>MAQVINTNSLSLLTQNNLNKSQSALGTAIERLSSGLRINSAKDDAAGQAIANRFTANIKGLTQASRNANDGISIAQTTEGALNEINNNLQRVRELAVQSANSTNSQSDLDSIQAEITQRLNEIDRVSGQTQFNGVKVLAQDNTLTIQVGANDGETIDIDLKQINSQTLGLDTLNVQQKYKVSDTAATVTGYADTTIALDNSTFKASATGLGGTDQKIDGDLKFDDTTGKYYAKVTVTGGTGKDGYYEVSVDKTNGEVTLAGGATSPLTGGLPATATEDVKNVQVANADLTEAKAALTAAGVTGTASVVKMSYTDNNGKTIDGGLAVKVGDDYYSATQNKDGSISINTTKYTADDGTSKTALNKLGGADGKTEVVSIGGKTYAASKAEGHNFKAQPDLAEAAATTTENPLQKIDAALAQVDTLRSDLGAVQNRFNSAITNLGNTVNNLTSARSRIEDSDYATEVSNMSRAQILQQAGTSVLAQANQVPQNVLSLLR[17x];>MASISSLGVGSNLPLDQLLTDLTKNEKGRLTPITKQQSANSAKLTAYGTLKSALEKFQTANTALNKADLFKSTVASSTTEDLKVSTTAGAAAGTYKINVTQLAAAQSLATKTTFATTKEQLGDTSVTSRTIKIEQPGRKEPLEIKLDKGDTSMEAIRDAINDADSGIAASIVKVKENEFQLVLTANSGTDNTMKITVEGDTKLNDLLAYDSTTNTGNMQELVKAENAKLNVNGIDIERQSNTVTDAPQGITLTLTKKVTDATVTVTKDDTKAKEAIKSWVDAYNSLVDTFSSLTKYTAVEPGEEASDKNGALLGDSVVRTIQTGIRAQFANSGSNSAFKTMAEIGITQDGTSGKLKIDDDKLTKVLKDNTAAARELLVGDGKETGITTKIATEVKSYLADDGIIDNAQDNVNATLKSLTKQYLSVSNSIDETVARYKAQFTQLDTMMSKLNNTSSYLTQQFTAMNKS[5x]

The flagellum is the most prominent extracellular structure in bacteria, with a molecular weight in the hundreds of megadaltons. Structurally, the flagellum can be divided into three major components: basal body, hook and filament. A ring-like structure formed by the proteins FlgK and FlgL, termed the hook–filament junction (HFJ), forms the connection between the flexible hook and the rigid filament. To assemble a filament, flagellin monomers are secreted through the flagellar basal body and hook, and polymerize at the distal end.

Here we report the structure of the filament cap complex in its native environment, assembled at the distal end of the flagellar filament. Three-dimensional (3D) classification identified the different states of the cap, resulting in a final 3.7-Å map resolving all five FliD subunits. The final cap model contains 5 FliD subunits and 17 copies of FliC in the filament; the HFJ model contains 13 copies of FlgE, 11 copies of FlgK and FlgL, and 14 copies of FliC. The flagellar cap complex is composed of five FliD subunits assembled into a pentamer with an overall shape resembling an acorn. The D2–D3 domains assemble into a star-shaped plane and the D0–D1 helices form a plug-like structure beneath. The D2–D3 plane and D0–D1 helices surround a large cavity, much larger than that described previously, and the D0 domains form an almost closed constriction in the secretion channel. All five FliD subunits show a pseudosymmetric arrangement, forming an asymmetric unit with three adjacent FliC molecules, labelled FliC 0, FliC +5 and FliC +6. Moreover, FliD 4 forms a substantially smaller interface with FliC +5. These unique features indicate that FliD 4 participates in the incorporation of a new FliC, which occurs in the gap between FliD 4 and FliC +6. During the incorporation of a FliC molecule, the D0–D1 domains of FliD 4 rise upwards (Δ = 25 Å) and shift in the clockwise (CW) direction (θ = 18°).>MATNTVYRINDRTSHHNLVRLNEPLPSVHGHEVLVEIRGVTLNARDIQICGGFYPAAAVKDNLVPCSDGAGVIAAVGDAVNDLEIGDRVIINISFDNLYGPLKSQKYMLGGGVDGTLRQYAAVPAHAIIKVPVDCKLDYVQLASLVCTGATVWNALYGYVPMKPGQTVLFQGTGGVSITGVQLAKAAGAVTIVTSSSDEKLEFVKDKFGVDHVINYKT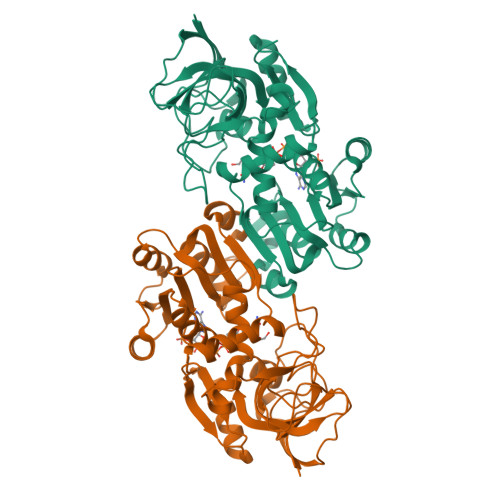TPNWAEEVRRFTNGEGADYVIEIGGAGTIEQSIQATASGGMIAVIGYLADIKQENMPNVPLLALIQGCALRGVQAGSKQLTTEMVNFVSRKNVQPYIHKTFGFTENEVMAAFDLQNSGKQIGKVGIAVKDQ[2x]> MWATLPLLCAGAWLLGVPVCGAAELCVNSLEKFHFKSWMSKHRKTYSTEEYHHRLQTFASNWRKINAHNNGNHTFKMALNQFSDMSFAEIKHKYLWSEPQNCSATKSNYLRGTGPYPPSVDWRKKGNFVSPVKNQGACGSCWTFSTTGALESAIAIATGKMLSLAEQQLVDCAQDFNNHGCQGGLPSQAFEYILYNKGIMGEDTYPYQGKD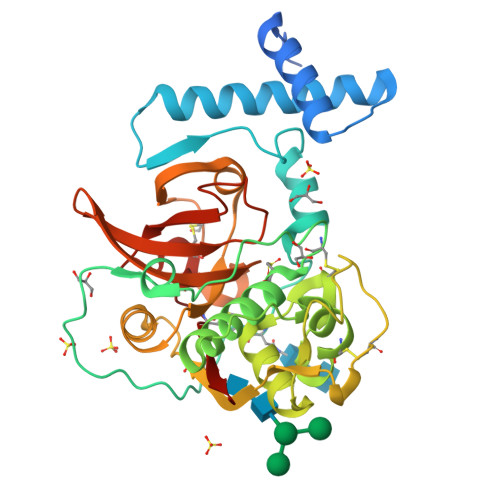GYCKFQPGKAIGFVKDVANITIYDEEAMVEAVALYNPVSFAFEVTQDFMMYRTGIYSSTSCHKTPDKVNHAVLAVGYGEKNGIPYWIVKNSWGPQWGMNGYFLIERGKNMCGLAACASYPIPLV4-methyl-3-[(1-methyl-6-pyrimidin-5-yl-pyrazolo[3,4-d]pyrimidin-4-yl)amino]-~{N}-[3-(trifluoromethyl)phenyl]benzamide | C25 H19 F3 N8 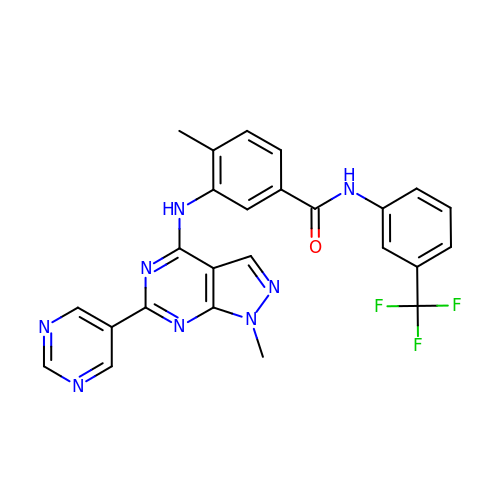O | QRWLLJMNPVOXLQ-UHFFFAOYSA-N>MEKTRPVHLWGTEEVAAWLEHLSLCEYKDIFTRHDIRGSGLLHLERRDLKDLGVTKVGHMKRILCGIKELSR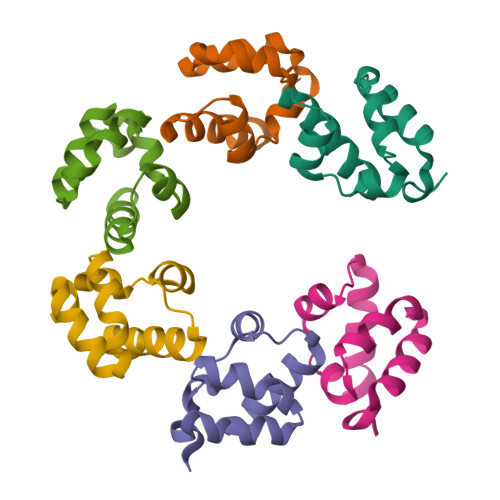SSRHHHHHH[6x]> MEAPPVTMMPVTGGTINMMEYLLQGSVLDHSLESLIHRLRGLCDNMEPETFLDHEMVFLLKGQQASPFVLRARRSMDRAGAPWHLRYLGQPEMGDKNRHALVRNCVDIATSENLTDFLMEMGFRMD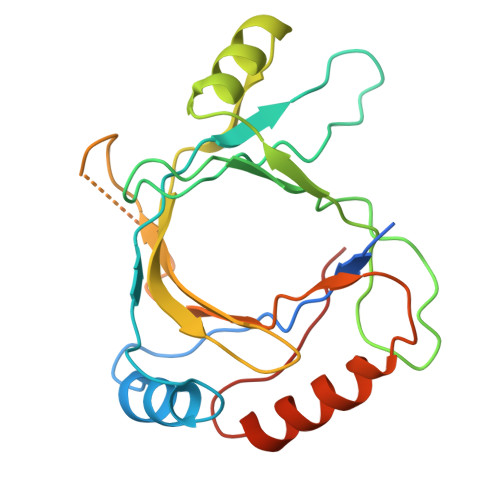HEFVAKGHLFRKGIMKIMVYKIFRILVPGNTDSTEALSLSYLVELSVVAPAGQDMVSDDMKNFAEQLKPLVHLEKIDPKRLM EndoBT-3987 is a secreted enzyme that initiates the HM degradation pathway and hydrolyzes the oligosaccharide from its polypeptide chain on the cell surface. ENGases are endoglycosidases that hydrolyze the chitobiose core of N-linked glycans (EC 3.2.1.96). Residues 26–41 were not visible in the structure. The full-length EndoBT-3987 comprises two domains from the N- to the C-terminus: (i) a β-sandwich domain (42–179) followed by a short linker (residues 180–193) that continues to (ii) a GH domain (residues 194–476). Here, we provide the high-resolution X-ray crystal structures of EndoBT-3987 in its unliganded form, in complex with its substrate, Man9GlcNAc2Asn, and two of its products, Man5GlcNAc and Man9GlcNAc.

EndoBT-3987 has a predicted signal peptide (residues 1–25; SignalP-5.0) that was removed from the construct. In order to obtain the crystal structure of the enzyme-substrate complex we used a catalytically inactive version of EndoBT-3987, in which the residues Asp312 and Glu314 are mutated to alanine and leucine, respectively (EndoBT-3987D312A/E314L; see below for further details). EndoBT-3987D312A/E314L-Man9GlcNAc2Asn crystallized in the R 3 space group with one molecule in the asymmetric unit and diffracted to a maximum resolution of 1.3 Å. The EndoBT-3987 GH domain adopts the conserved (α/β)8-barrel topology typical of enzymes from the GH18 family, with a shallow pocket in which one molecule of the Man9GlcNAc2Asn substrate is unambiguously identified in the crystal structure. Specifically, the Man9GlcNAc2Asn substrate is located in the center of the (α/β)8-barrel, flanked by the connecting loops β10–α2 (loop 1; residues 201–205), β11–α3 (loop 2; residues 228–245), β14–α4 (loop 3; residues 275–286), β15–α5 (loop 4; residues 313–330), β16–β17 (loop 5; residues 355–374), β17– β18 (loop 6; residues 379–395), β18–α6 (loop 7; residues 402–411), and β19–α7 (loop 8; residues 430–432). The GlcNAc (−1) residue is in a skew boat conformation (1S5), with the C2-acetamido group pointed toward the mutated catalytic residue D312A. The skew boat conformation of GlcNAc (−1) is stabilized by hydrogen bonds between the O3 atom and the side chain of Y315, the N2 atom of the acetamide group and the side chain of Y380, and the O6 atom and the side chain of E401. The Manα1–2Manα1–6(Manα1–2Manα1–3)Manα1–6 antenna (antenna 1), mainly interacts with loops 1, 2, 3, and 4, whereas the Manα1–2Manα1–2Manα1–3 antenna (antenna 2) interacts with loops 1 and 7. The O2 atom of Man (−3), which bisects antenna 1 into two additional sub-antennae, antenna α1,6′ (antenna 1a; Man (−4) and (−5) residues), and antenna α1,3′ (antenna 1b; Man (−6) and (−7) residues; Fig. 2), makes a hydrogen bond with the Nε2 atom of H277.

> GDDLEVGKNIDESAYSGIYENNAYLRDGKSNLVSKVVELHGETYATTVKMGLSKTPNTATSAKVKIDAAYLETYNKAHNTDFALYPQDLVTFANEGILTVNANTKSAEVEMTIRAGEGLQEDKTYAIPVAISDQSSDITIKDEDAKHCIYLVKDMRNAGDAYKGEGVMQGYLFFEVNDVNPLNTLSFQLENGKLLWDVVVLFAANINYDAEAGRPRVQCNPNVQYLLDNNETLLQPLRRRGVKVLLGLLGNHDITGLAQLSEQGAKDFAREVAQYCKAYNLDGVNYADLYSNSPDLSNPSLTNPSTAAAARLCYETKQAMPDKLVTVFDWGQMYGVATVDGVDAKEWIDIVVANYGSAAYPIGQMTKKQCSGISMEFNLGGGGSLSASKAQSMIDGGYGWFMGFAPSPAKYGSVFSRLQGGGEVLYGSNVAAPTIFYKKNDPTPYKYPDDL[(2~{R})-4-(phenylmethyl)morpholin-2-yl]methanol | 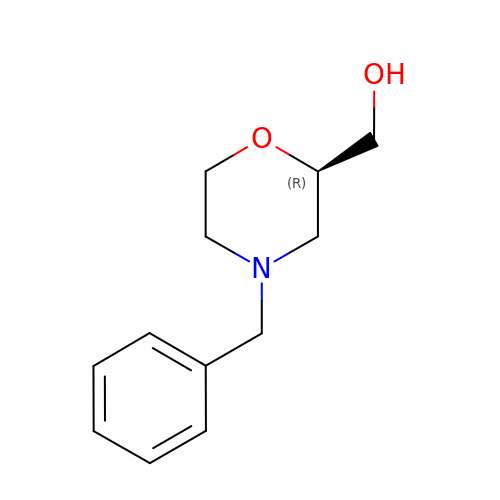C12 H17 N O2 | WQNIKIMRIXHNFF-GFCCVEGCSA-N2-AMINO-5-HYDROXY-BENZIMIDAZOLE | C7 H7 N3 O | 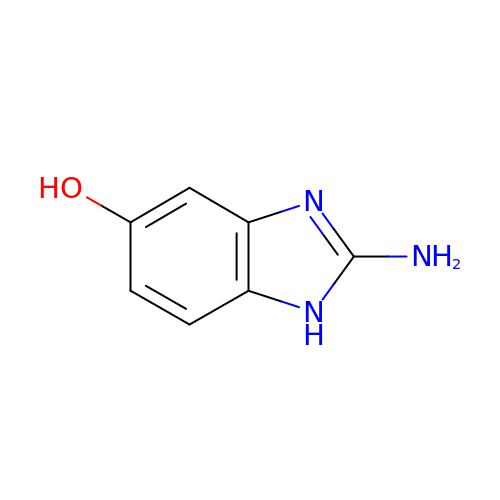FNSYWIPPPFVBAV-UHFFFAOYSA-N> AEDFVSENSNNKRAPYWTNTEKMEKRLHAVPAANTVKFRCPAGGNPMPTMRWLKNGKEFKQEHRIGGYKVRNQHWSLIMESVVPSDKGNYTCVVENEYGSINHTYHLDVVERSPHRPILQAGLPANAST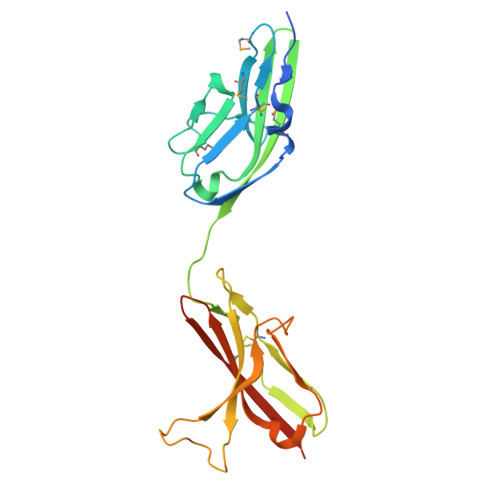VVGGDVEFVCKVYSDAQPHIQWIKHVEKNGSKYGPDGLPYLKVLKHSGINSSNAEVLALFNVTEADAGEYICKVSNYIGQANQSAWLTVLPKQQAPGREKE> SVNLDVKHFSPEELKVKVLGDVIEVHGKHEERQDEHGFISREFHRKYRIPADVDPLTITSSLSSDGVLTVNGPRKQVSGPERTIPI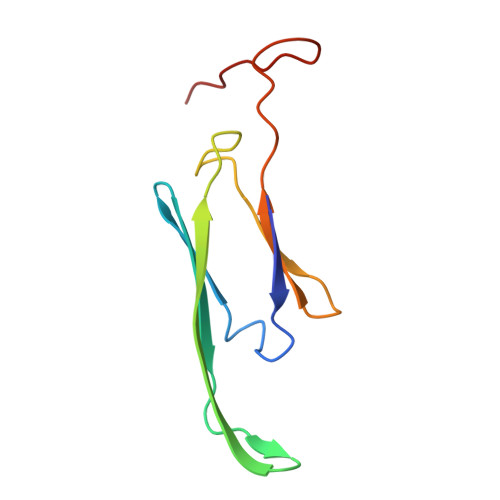TR>CGCGA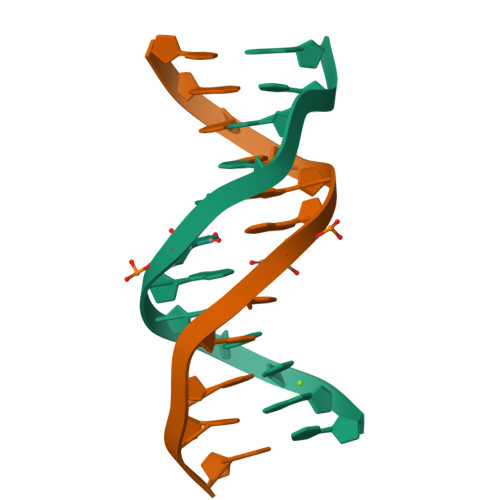AUTCGCG[2x]>CPRFLKVKNWETEVVLTDTLHLKSTLETGCTEYICMGSIMHPSQHARRPEDVRTKDQLFPLAKEFIDQYYSSIKRFGSKAHMERLEEVNKEIDTTSTYQLKDTELIYGAKHAWRNASRCVGRIQWSKLQVFDARDCTTAHGMFNYICNHVKYATNKGNLRSAITIFPQRTDGKHDFRVWNSQLIRYAGYKQPDGSTLGDPANVQFTEICIQQGWKPPRGRFDVLPLLLQANGNDPELFQIPPELVLEVPIRHPKFEWFKDLGLKWYGLPAVSNMLLEIGGLEFSACPFSGWYMGTEIGVRDYCDNSRYNILEEVAKKMNLDMRKTSSLWKDQALVEINIAVLYSFQSDKVTIVDHHSATESFIKHMENEYRCRGGCPADWVWIVPPMSGSITPVFHQEMLNYRLTPSFEYQPDPWNTHVWK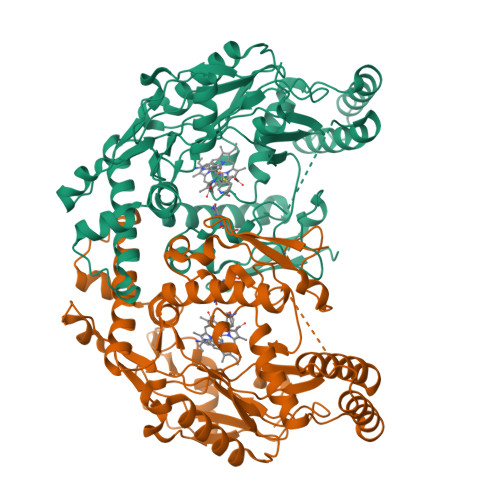[2x]>[2x]AGPTAVPLGTAGNYAILASYAVSTVPQSAITGAVGISPAAGTFLTGFSLTMSGTGTFSTSTQVTGQLTAA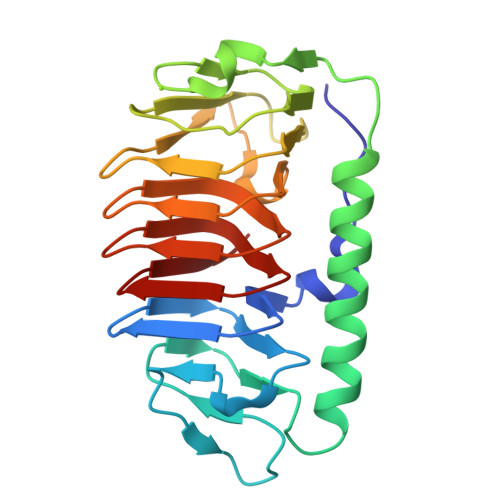DYGTPTPSILTTAIGDMGTAYTNGATRSGPDFLEIYTGALGGTTLLPGLYKWTSSVGASADFTISGTSTDTWIFQIDGTLGLAAGKKITLAGGAQAKNIIWVVAGAVSIEAGAQFEGVILAKTAVTLKTGSSLNGRILAQTSVALQSATVVQK>GPETQELASKRVDIQNKRFYLDVKQNAKGRFLKIAEVGAGGNESRLTLSMSVAVEFRDYLGDFIEHYAQLGPSQPPDLAQAQDEPRRALKSEFLVRENRKYYMDLKENQRGRFLRIRQTVNRGPGLGSTQGQTIALPAQGLIEFRDALAKLIDDYGVE[2x]

Mutations in the human PURA gene cause the neurodevelopmental PURA syndrome. Based on the crystal structures of PURA from Drosophila melanogaster (dmPURA), three conserved sequence regions termed PUR repeats I, II, and III were identified to fold into globular domains. Whereas PUR repeat I and II assemble into an N-terminal PUR domain via intramolecular interactions, two C-terminal PUR repeats III from different molecules interact with each other and thus mediate dimerization of PURA. All these PUR domains belong to the class of the PC4-like protein family, which mainly bind single-stranded nucleic acids and can unwind double-stranded DNA and RNA.

In contrast, the spectrum for hsPURA I–II K97E indicated a strongly altered secondary structure content. To understand how exactly the surface-exposed K97E mutation alters the domain folding of PURA, we solved the crystal structure of hsPURA I–II K97E. The asymmetric unit of the crystal contained two molecules of hsPURA I–II K97E and showed good overall fold similarity to the hsPURA I–II structure. However, an overlay of both molecules of the K97E-variant protein from the asymmetric unit also revealed unusual differences between them with r.m.s.d. of 1.48 Å for 125 superimposed Cα atoms. More C-terminally, the loop linking β6 and β7 is shorter by two residues, thereby correcting again the sequence register within the next β-strands (β7 and β8). From all the areas of the structure, the β-ridge appears to be structurally the most divergent part. It is surprising that the K97E point mutation, which is located on the β4 strand of the β-ridge, induces the observed unusual change in the β-sheet arrangement without destroying the domain’s overall scaffold. Importantly, all the resonances perturbed upon K97E mutation remained in the presence of 1H-saturation, confirming that the structural rearrangement does not induce protein unfolding. Together, this shows that the K97E mutation does not induce global unfolding of hsPURA I–II, but rather triggers structural rearrangements mostly in the β-strand region. While hsPURA I–II quantitatively bound a 24-mer CGG-repeat RNA, the hsPURA I–II K97E-variant protein showed moderately but significantly decreased RNA binding. With an effect considerably stronger than observed for RNA binding, the hsPURA I–II K97E variant showed a loss of strand-separation activity by 90%.>[3x]MGDGANSDAAKEYLTKDSFSYEVYGIIAMQAAYRDYDSGDAKQDDNLGGMQLNNESRIGFRGKKQFANFEPTFIWQIEGGYVDPSFGGEGAGLGERDTFVGFESASWGQVRLGRVLTPMYELVDWPASNPGLGDVYDWGGAIGGAKYQDRQSNTIRWDSPMYADKFSIDAAVGAGDKAGLGAGDDYWGGIAAHYKLGPLQLDAAYEGNRNIEAEGQTWENNTYLVGVQGWFENGISFFAQYKYME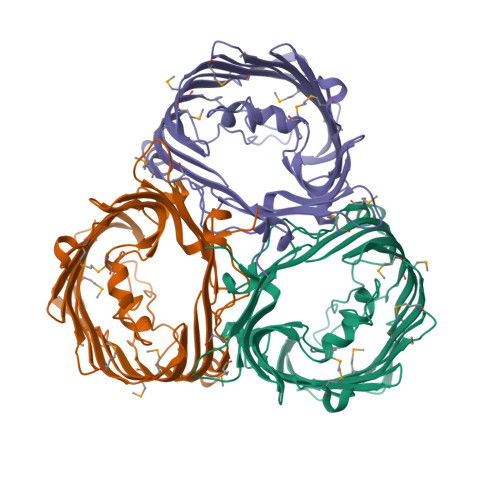ADASNGVNEKQDAMSAGLMYTTGDWQYKLGYAANFDLERDGKTLSNTSDDVVSAQIMYFVDPSAVLYARARMNDFNEGLDGLDDAARWTSGTNGDYNEYSVGVEYYF> XADVAGTSNRDFRGREQRLFNSEQYNYNNSLNGEVSVWVYAYYSDGSVLVINKNSQYKVGISETFKKPRAIQIIFSPSVNVRTIKMAKGNAVSVPDEYLQRSHPWEATGIKYRKIKRDGEIV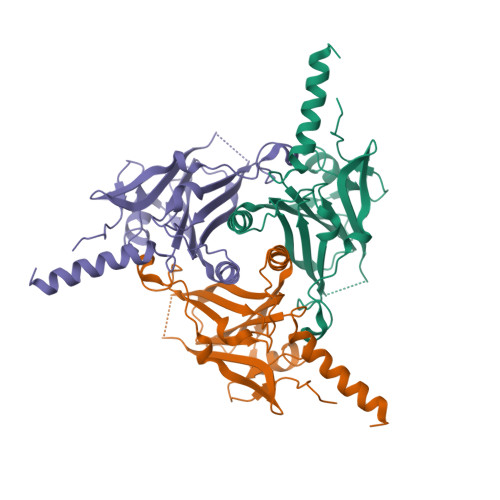GYSHYFELPHEYNSISLAVSGVHKNPSSYNVGSAHNVMDVFQSCDLALRFCNRYWAELELVNHYISPNAYPYLDINNHSYGVALSNRQ The cyanobacterial enzyme CylK assembles the cylindrocyclophane natural products by performing two unusual alkylation reactions, forming new carbon–carbon bonds between aromatic rings and secondary alkyl halide substrates. Two molecules of 1 are then dimerized by an alkyl chloride-utilizing enzyme, CylK, via the formation of two new carbon–carbon (C–C) bonds to construct a paracyclophane ring system (Nakamura et al., 2017). The structure reveals an unprecedented fusion of two protein folds, an N-terminal Ca2+-binding domain and a C-terminal β-propeller domain. We identified the active site of CylK at the interface of its N- and C-terminal domains.

CylK crystallized in the C2221 space group with a single monomer in the asymmetric unit. Phase information was obtained by partial substitution of native Ca2+-binding sites in CylK with Tb3+, followed by collection of X-ray diffraction datasets at the Tb X-ray absorption peak energy. The structure of CylK was solved to 1.68 Å resolution via a combined MR and single-wavelength anomalous diffraction (SAD) approach, with the MR search model generated from a poly-alanine seven-bladed β-propeller. The modified β-roll structure in CylK contains three vertically aligned Ca2+ ions on one side of the core fold. Also, the loops that connect subsequent blades contain unique blade-bridging Ca2+-binding sites, suggesting a shared role for this divalent metal in structural stabilization of both domains of CylK. Cavity 1 is lined by the top face of the β-propeller domain and the N-terminal domain, forming a solvent-accessible tunnel that is ~18 Å deep and 15 Å wide at its largest point. Although 3 was required for CylK crystallization, we could not model the alkyl resorcinol substrate in the resulting structure. Notably, the apo CylK model also contained a positive Fo−Fc electron density peak at the Br1 site. Given the presence of chloride salts in the protein storage buffer, we modeled this site as a chloride ion in the apo model. However, the closest Ca2+ ion is approximately 8 Å from this pocket.

> MKKNKKTTKSLLSADEKITESLRSTLSDVLPDQLQTYIRTVLQFSGRPEGANLLTGPNTEIEFFSQDPNKNFPNIFAKYSNVLTVSSDPNFITSEDEEVKIIWGRHGSDSLIGFDPGADLVGKRRIDIFLGDFIDEQFNPIPGALNAGKSWSDRFILGDWQKPYYFEDDETLGLNQSAMILDFNPNEDVIQLHGDRQDYELVNISLGTAIFWREKKGYDLIGVLGGVSDLSLKGDYFEFKGNTAPKTVLKTAEHIGTAANDYIFSSTVDAKGNFYVGGGTGGSLGGRNIGARDAWLAKYDSNGNQRWSRQFGSTGTESLWGMASDGSNIYVAGNTTGQLENNTVKGGNDAYLAKYDSDGNQVWIKQNGTYTLEESYKITVDSSGNIYTAGHTFGSLGGPNQNLEQGEVFELPSTDGYVAKFDSNGNQLWVAQFGTITLDDNWGVAADNNGNVFAGGNTKGSFGAKNTGTAGEYDAWLVKLNKDGQTDWVRQFGTPNYDFMWDIETDSLGDIYATGWTLGDLGGKNAGSYDVWLAKYNTNGNQLWIKQFGTSEDDAPFLDGIDIDANDNIFLTGNTNGNLGGANAGSYDAWAAKFDKDGNQLWLKQFGTPDYDTATTVTAVNFGKLYVSGITEGSLGTTNAGSYDSWALKLDADNGEIQDFNSSTNTFGQTGFLNLGSAWSHPQFEK>AGASRQRKLEALIRDPRSPINVESLLDGLNSLVLDLDFPALRKNKNIDNFLNRYEKIVKKIRGLQMKAEDYDVVKVIGRGAFGEVQLVRHKASQKVYAMKLLSKFEMIKRSDSAFFWEERDIMAFANSPWVVQLFYAFQDDRYLYMVMEYMPGGDLVNLMSNYDVPEKWAKFYTAEVVLALDAIHSMGLIHRDVKPDNMLLDKHGHLKLADFGTCMKMDETGMVHCDTAVGTPDYISPEVLKSQGGDGFYGRECDWWSVGVFLYEMLVGDTPFYADSLVGTYSKIMDHKNSLCFPEDAEISKHAKNLICAFLTDREVRLGRNGVEEIRQHPFFKNDQWHWDNIRETAAPVVPELSSDIDSSNFDDIEDDKGDVETFPIPKAFVG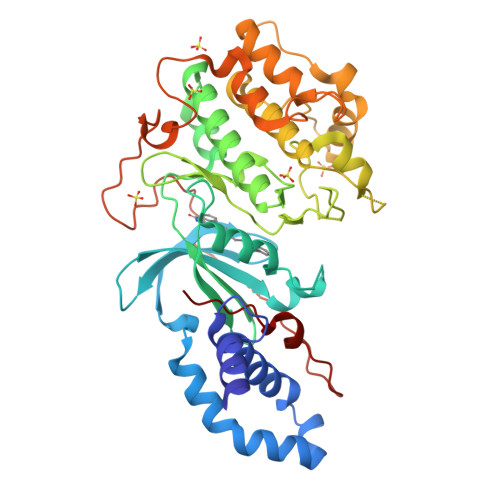NQLPFIGFTYYR[4x]> GPSSSKSEENISLVYEIDGTEALGSCLRVRPCSNDAPDLSKCTIQWYRSSSDGSKKELISGATKSVYAPEPFDVGRVLHADIIYDGHSLSLSTVGKIDPAAGLGSYVEALVRKHDVDFNVVVTQMSGEDHTSESIHLFHVGKMRIKLCKGKTVIAKEYYSSAMQLCGVRGGGNAAAQALYWQAKKGVSFVIAFESERERNAAIMLARRFACDCNV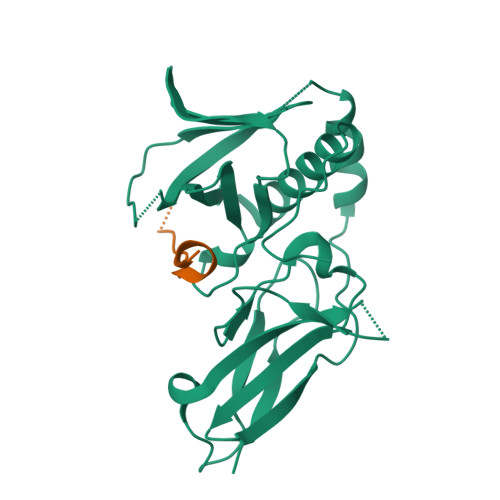TLAGPEDRTETGQSP;> GGSDPAISKDVVLSSSSFLRA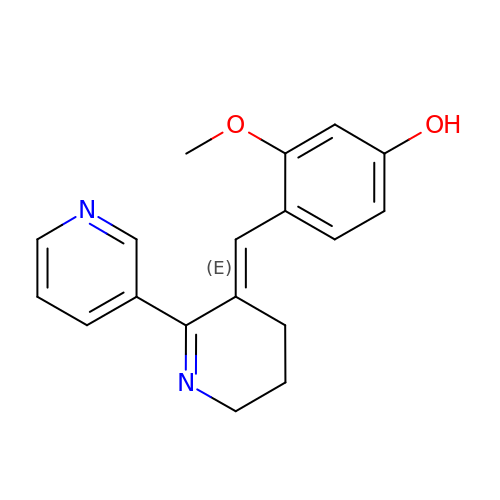4-[(E)-5,6-DIHYDRO-2,3'-BIPYRIDIN-3(4H)-YLIDENEMETHYL]-3-METHOXYPHENOL | C18 H18 N2 O2 | KXAAIPFSUGPVMQ-GXDHUFHOSA-N> MDEFEMIKRNTSEIISEEELREVLKKDEKSAHIGFEPSGKIHLGHYLQIKKMIDLQNAGFDIIILLADLAAYLNQKGELDEIRKIGDYNKKVFEAMGLKAKYVYGSEFQLDKDYTLNVYRLALKTTLKRARRSMELIAREDEN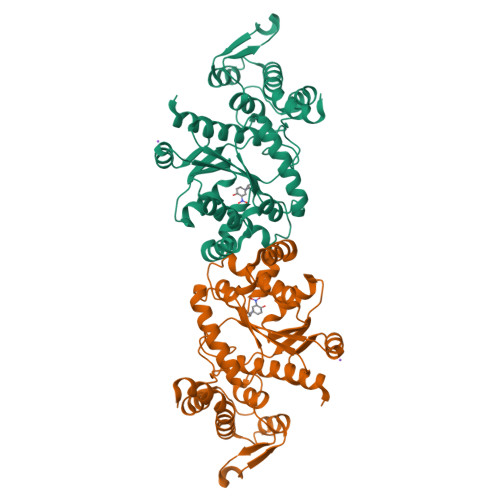PKVAEVIYPIMQVNSAHYRGVDVAVGGMEQRKIHMLARELLPKKVVCIHNPVLTGLDGEGKMSSSKGNFIAVDDSPEEIRAKIKKAYCPAGVVEGNPIMEIAKYFLEYPLTIKRPEKFGGDLTVNSYEELESLFKNKELHPMDLKNAVAEELIKILEPIRKRLLEHHHHHH> MYYGISQFSEAYNKILRNSSSHSSCQLVIFVSCLNIDALCATKMLSLLFKKQLVQSQIVPIFGYSELRRHYSQL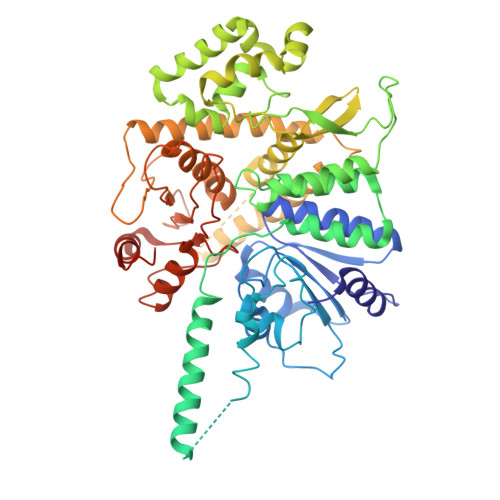DDNINSLLLVGFGGVIDLEAFLEIDPQEYVIDTDEKSGEQSFRRDIYVLDAHRPWNLDNIFGSQIIQCFDDGTVDDTLGEQKEAYYKLLELDEESGDDELSGDENDNNGGDDEATDADEVTDEDEEDEDETISNKRGNSSIGPNDLSKRKQRKKQIHEYEGVLEEYYSQGTTVVNSISAQIYSLLSAIGETNLSNLWLNILGTTSLDIAYAQVYNRLYPLLQDEVKRLTPSSRNSVKTPDTLTLNIQPDYYLFLLRHSSLYDSFYYSNYVNAKLSLWNENGKKRLHKMFARMGIPLSTAQETWLYMDHSIKRELGIIFDKNLDRYGLQDIIRDGFVRTLGYRGSISASEFVEALTALLEVGNSTDKDSVKINNDNNDDTDGEEEEDNSAQKLTNLRKRWVSNFWLSWDALDDRKVELLNRGIQLAQDLQRAIFNTGVAILEKKLIKHLRIYRLCVLQDGPDLDLYRNPLTLLRLGNWLIECCAESEDKQLLPMVLASIDENTDTYLVAGLTPRYPRGLDTIHTKKPILNNFSMAFQQITAETDAKVRIDNFESSIIEIRREDLSPFLEKLTLSGLLDYKDHDGDYKDHDIDYKDDDDK4,6-dimethyl-N'-(3-pyridin-2-ylisoquinolin-1-yl)pyrimidine-2-carboximidamide 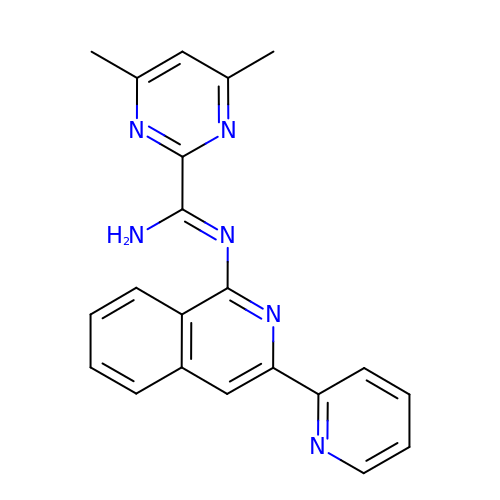| C21 H18 N6 | YKSJLEVXPOMXPZ-UHFFFAOYSA-N> QCFLIDKNFVNKAVESANLTKDDVVLEIGLGKGILTEELAK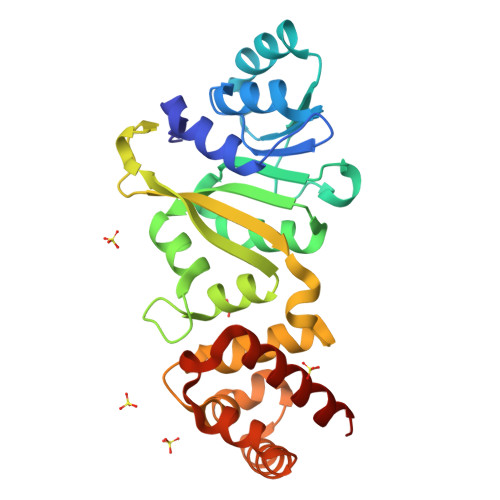NAKKVYVIEIDKSLEPYANKLKELYNNIEIIWGDALKVDLNKLDFNKVVANLPYQISSPITFKLIKRGFDLAVLMYQYEFAKRMVAAAGTKDYGRLSVAVQSRADVEIVAKVPPSAFYPKPKVYSAIVKIKPNKGKYHIENENFFDDFLRAIFQHRNKSVRKALIDSSKELNYNKDEMKKILEDFLNTNSEIKNLINEKVFKLSVKDIVNLSNEFYRFLQNR>[8x]MGSSHHHHHHSSGRENLYFQGMTLKAGIVGIGMIGSDHLRRLANTVSGVEVVAV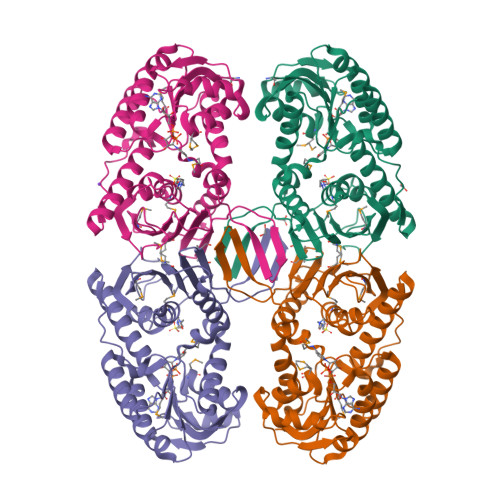CDIVAGRAQAALDKYAIEAKDYNDYHDLINDKDVEVVIITASNEAHADVAVAALNANKYVFCEKPLAVTAADCQRVIEAEQKNGKRMVQIGFMRRYDKGYVQLKNIIDSGEIGQPLMVHGRHYNASTVPEYKTPQAIYETLIHEIDVMHWLLNEDYKTVKVYFPRQSSLVTTLRDPQLVVMETTSGINIVVEVFVNCQYGYDIHCDVTGEKGMAELPTVASAAVRKAAKYSTDILVDWKQRFIDAYDIEFQDFFDRLNAGLPPAGPTSWDGYLAAVTADACVKSQETGNTEIVELPSKPDFYK> HMVPACPPPNPHQVEQLQDFVSQSQRLFVMTGAGISTESGIPDYRSEGVGLYSRTERRPIQHS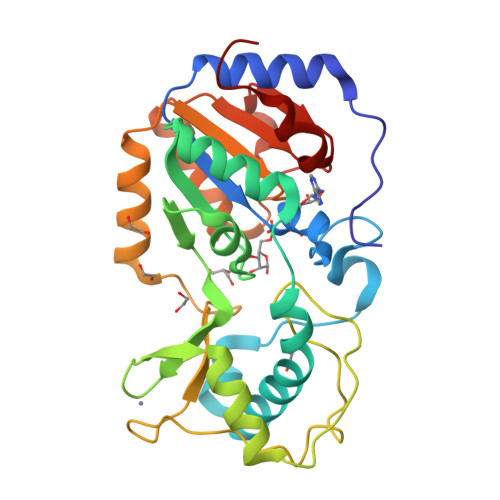EFVQSQAARRRYWARNFVGWPSFSSHEPNSAHVNLCKWERAGRLHWLVTQNVDALHTKAGQCRLSELHGCTHRVICLGCQTVTKRSELQERFLNLNPSWNEQAHGLAPDGDVFLTDEQVSDFQVPACTKCGGILKPQVTFFGDTVNRGFVFSIYEQMKQADAMLIVGSSLQVYSGYRFALNAKELHLPIAILNIGPTRADHLAKVKVSARCGDVLPHILLQDQ> HHHHHHSQDPMNALTTIDFNQHVIVRLPSKNYKIVELKPNTSVSLGKFGAFEVNDIIGYPFGLTFEIYYDGEEVSSDENRDSKPKNKIPIGKVRLLSQEIKDVNNDKDDGQSEPPLSIKEKSVSLELSSIDSSATNQNLVNMGSKAQELTVEEIEKMKQESLSSKEIIDKIIKSHKSFHNKTVYSQEKYVNRKKQKFAKYFTVEYLSSSNLLQFLIDKGDIQRVLDMSQESMGMLLNLANIQSEGNYLCMDETGGLLVYFLLERMFGGDNESKSKGKVIVIHENEHANLDLLKFANYSEKFIKEHVHTISLLDFFEPPTLQEIQSRFTPLPKEEARALKGGKKNSYYRKLRWYNTQWQILELTGEFLYDGLVMATTLHLPTLVPKLAEKIHGSRPIVCYGQFKETLLELAHTLYSDLRFLAPSILETRCRPYQSIRGKLHPLMTMKGGGGYLMWCHRVIPAPEPVSENATAADSSEKLAEHGAKKQKI;> MSTNCFSGYKDLIKEGDLTLIWVSRDNIKPVRMHSEEVFNTRYGSFPHKDIIGKPYGSQIAIRTKGSNKFAFVHVLQPTPELWTLSLPHRTQIVYTPDSSYIMQRLNCSPHSRVIEAGTGSGSFSHAFARSVGHLFSFEFHHIRYEQALEEFKEHGLIDDNVTITHRDVCQGGFLIKKGDTTSYEFGNNETAASLNANVVFLDLPAPWDAIPHLDSVISVDEKVGLCCFSPCIEQVDKTLDVLEKYGWTDVEMVEIQGRQYESRRQMVRSLNDALERLRDIKRHKLQGVERRKRMFNNTIDSNDEKVGKRNEDGVPLTEKAKFNPFGKGSRIKEGDSNYKWKEVTKMEAEIKSHTSYLTFAFKVVNRSRDDEKVNEILRSTEK

Adenine at position 58 (A58) located in the T-loop is one of the most conserved nucleosides in tRNA, and the occurrence of 1-methyladenosine (m1A) at position 58 has been reported from all three kingdoms7. In yeast, the two subunits complex TRM6-TRM61 has been identified as the key factor of this methyl transfer reaction. In this study, we report the crystal structures of S.cerevisiae TRM6-TRM61 holoenzyme and TRM6-TRM61 in complex with SAM. TRM6 and TRM61 adopt a similar fold, with a high structural similarity to the prokaryotic counterpart TrmI.

To improve understanding the target tRNA recognition and catalytic mechanism of the two component m1A58 tRNA methyl- transferase in eukaryotes, we solved the structure of the TRM6-TRM61 holoenzyme from S. cerevisiae by the SAD method using the Se anomalous signal. The final model has been refined to 2.2 Å resolution and the details of the data collection and refinement statistics are summarized in Table 1. One TRM6-TRM61 heterodimer adopts a rectangular shape with two arms protruding from the core. Previously, we have shown that a symmetric unit of the TRM6-TRM61 crystal contains one molecule of TRM6 and one molecule of TRM61, forming a 1:1 heterodimer. Further examination of symmetry- related molecules indicated that TRM6 and TRM61 form a 2:2 tetrameric heterocomplex, displaying a “Ω“ shape. The TRM6-TRM61 holoenzyme eluted with a molecular weight of approximately 219.5 kDa, which is very close to the theoretical value of 196.6 kDa for the TRM6-TRM61 heterotetramer. In the structure of apo TRM61, loop β7/α4 and loop α2/α3 lock the binding pocket for the homocysteine moiety of SAM. In the structure of apo S. cerevisiae TRM6-TRM61, the residues 88–188 located at the N-terminal β-barrel domain of TRM6 are not visible due to the flexibility. In addition, the arm insertion between β10 and β11 of TRM6 in the apo S. cerevisiae TRM6-TRM61 protrudes away from the position that is suitable for recognizing the anticodon arm of the substrate tRNA. In the tRNA-unbound state, the TRM6-TRM61 holoenzyme likes an open hand, which creates enough space for the entrance of target tRNA.> AIPAPTDLKFTQVTPTSLSAQWTPPNVQLTGYRVRVTPKEKTGPMKEINLAPDSSSVVVSGLMVATKYEVSVYALKDTLTSRPAQGVVTTLENVSPPRRARVTDATETTITISWRTKTETITGFQVDAVPANGQTPIQRTIKPDVRSYTITGLQPGTDYKIYLYTLNDNARSSPVVIDASTAIDAPSNLRFLATTPNSLLVSWQPPRAR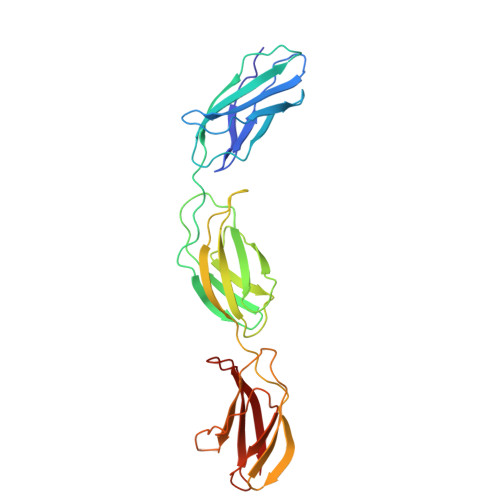ITGYIIKYEKPGSPPREVVPRPRPGVTEATITGLEPGTEYTIYVIALKNNQKSEPLIGRKKT>MGSDKIHHHHHHMNNTIPRWRGFNLLEAFSIKSTGNFKEEDFLWMAQWDFNFVRIPMCHLLWSDRGNPFIIREDFFEKIDRVIFWGEKYGIHICIS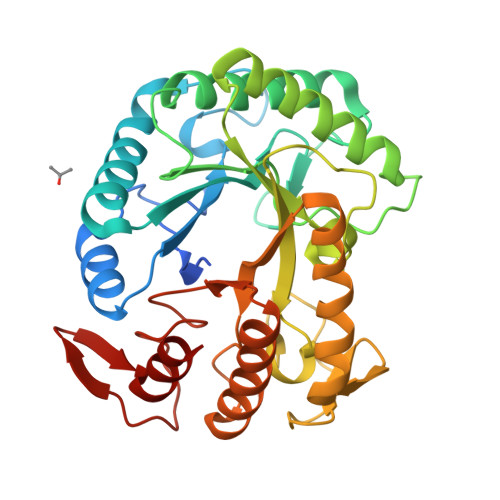LHRAPGYSVNKEVEEKTNLWKDETAQEAFIHHWSFIARRYKGISSTHLSFNLINEPPFPDPQIMSVEDHNSLIKRTITEIRKIDPERLIIIDGLGYGNIPVDDLTIENTVQSCRGYIPFSVTHYKAEWVDSKDFPVPEWPNGWHFGEYWNREKLLEHYLTWIKLRQKGIEVFCGEMGAYNKTPHDVVLKWLEDLLEIFKTLNIGFALWNFRGPFGILDSERKDVEYEEWYGHKLDRKMLELLRKY[2x]>[2x]MTGGMKPPARKPRILNSDGSSNITRLGLEKRGWLDDHYHDLLTVSWPVFITLITGLYLVTNALFALAYLACGDVIENARPGSFTDAFFFSVQTMATIGYGKLIPIGPLANTLVTLEALCGMLGLAVAASLIYA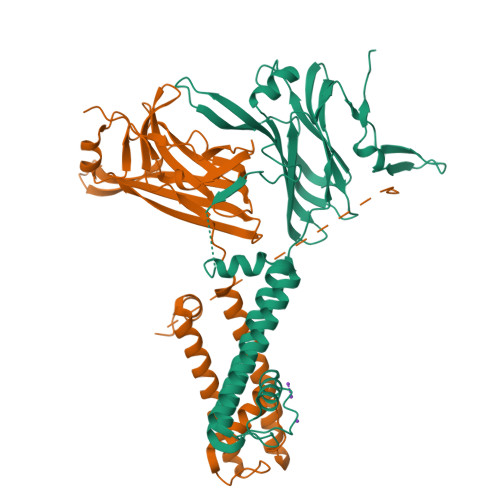RFTRPTAGVLFSSRMVISDFEGKPTLMMRLANLRIEQIIEADVHLVLVRSEISQEGMVFRRFHDLTLTRSRSPIFSLSWTVMHPIDHHSPIYGETDETLRNSHSEFLVLFTGHHEAFAQNVHARHAYSCDEIIWGGHFVDVFTTLPDGRRALDLGKFHEIAQHHHHHH Danazol | C22 H27 N O2 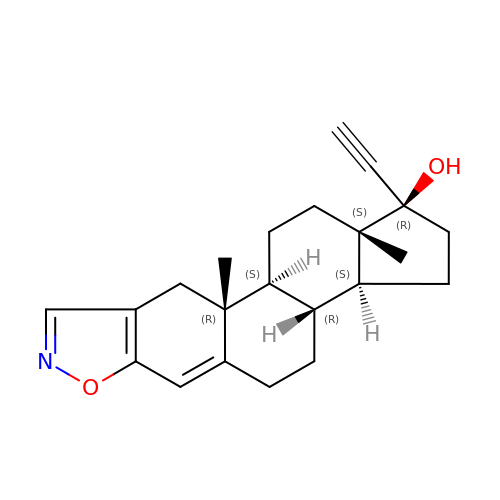| POZRVZJJTULAOH-LHZXLZLDSA-N> MNQGGVFPLPFKIAGLGRYVPADVVLSSDLEKKYDLPPGWCVEKQGIRERRWVKDETASFMGAEAAKEAVRDAGLKLEDIDLIINASGSPEQAVPDGGPLVQRELGLGRSGVPSITVNASCLSFFVALDVAANYLNMRRYKRILIVSSDISSVALDFRKPENFTLFGDAAAAAVVTLPEPGEKSCIHASQVRTYGYGAEFSMVPGGGSRRHPNGKNTTPEDNYLHMNGAELLKIGFEYLPRFNEALWKQCPDITIKDCRYVIPHQPSRVVLDYLSLTYPDDKLVRIIDRFANCIGASMPMALY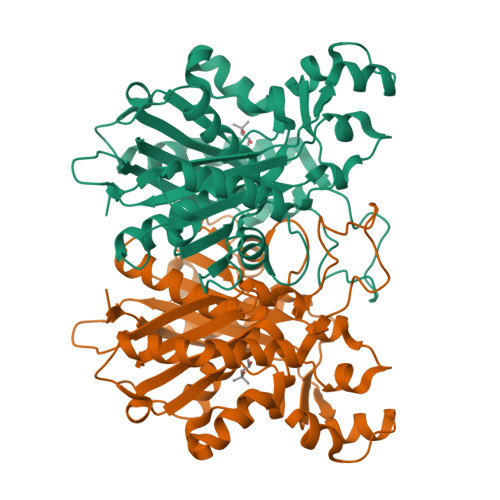EAVKVGGLRRGERGVLTGTGSGVSFVGMVFTY>[2x]MAVESRVTQEEIKKEPEKPIDREKTCPLLLRVFTTNNGRHHRMDEFSRGNVPSSELQIYTWMDATLKELTSLVKEVYPE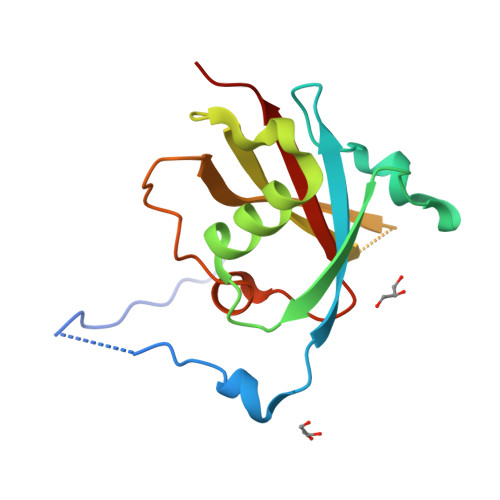ARKKGTHFNFAIVFMDLKRPGYRVKEIGSTMSGRKGTDDSMTLQSQKFQIGDYLDIAITPPNRA> MAEEEEVEEGRSSSSAILDLPEPLLLHILSFLTDVRSRHRAALACGRMRAAERATRSELSLRGDPRSPGFLFLSHAFRFPALEHLDLSLVSPWGHPLLSSVPPCGGGGGGAPSASSSSGMNVYHPEAISEQNAFIAARLAGCFPAVTSLAVYCRDPTTLANLTPHWQASLRRVKLVRWHQRPPTLPDGADLEPLLETCAALRELDLSEFYCWTEDVVRALTTHPSATAALTHLDLGLAAATDGFKSSELGPIAASCPNLRKLVAPCLFNPRFSDCVGDDALLSLATSCPRLTVLRLSEPFEAAANIQREEAAITVAGLVAFFAALPALEDFTMDLQHNVLEAAPAMEALARRCPRIKFLTLGSFQGLCKASWLHLDGVAVCGGLESLYMKNCQDLTDASLAAIGRGCRRLAKFGIHGCDLVTSAGIRRLAFTLRPTLKEVTVLHCRLLHTAECLTALSPIRDRIESLEINCVWNTTEQPCSVANGTTTECDPEDDELGEVYESAAKKCRYMEFDDLGSWEMLRSLSLWFSAGQLLSPLISAGLDSCPVLEEISIKVEGDCRTCPRPAPRTIFGLSDLAGFPVLAKMKLDLSEAVGYALTAPTGQMDLSLWERFYLHGI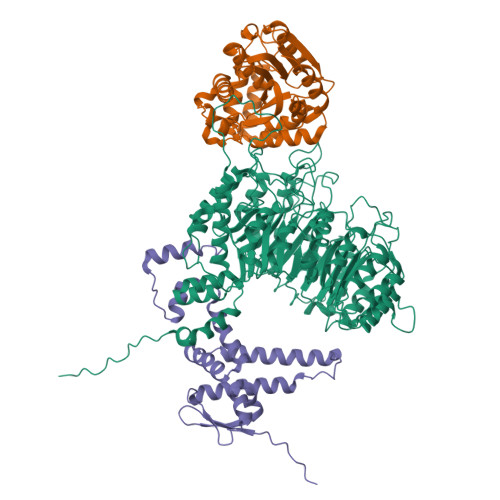ESLQTLYELDYWPPQDKDVHHRSLTLPAVGLIQRCVGLRKLFIHGTTHEHFMTFFLSIPNLRDMQLREDYYPAPENDLMFTEMRAESWLRFEVQLNSRQIDD;> MAAEAETKAMITLRSCEGQVFEVAEAVAMESQTIRHMIEDKCADTGIPLPNVSAKILSKVIEYCSKHVEARGGAAAAADGDAPAPAAVEANKAVEDELKTFDAEFVKVDQSTLFDLILAANYLNIKGLLDLTCQTVADMIKGKTPEEIRKTFNIKNDFTPEEEEEVRRENQWAFE;> MLRSTHPPPSSPSSSSSGGGGGGGSSASSSSEKTMVGGGGGGGGGSGSAAPSGAKLLQILNVRVVGSGERVVVLSHGFGTDQSAWSRVLPYLTRDHRVVLYDLVCAGSVNPDHFDFRRYDNLDAYVDDLLAILDALRIPRCAFVGHSVSAMIGILASIRRPDLFAKLVLIGASPRFLNDSDYHGGFELEEIQQVFDAMGANYSAWATGYAPLAVGADVPAAVQEFSRTLFNMRPDISLHVCQTVFKTDLRGVLGMVRAPCVVVQTTRDVSVPASVAAYLKAHLGGRTTVEFLQTEGHLPHLSAPSLLAQVLRRALARY> SDSLSKSPENWMSKLDDGKHLTEINIPGSHDSGSFTLKDPVKSVWAKTQDKDYLTQMKSGVRFFDIRGRASADNMISVHHGMVYLHHELGKFLDDAKYYLSAYPNETIVMSMKKDYDSDSKVTKTFEEIFREYYYNNPQYQNLFYTGSNANPTLKETKGKIVLFNRMGGTYIKSGYGADTSGIQWADNATFETKINNGSLNLKVQDEYKDYYDKKVEAVKNLLAKAKTDSNKDNVYVNFLSVASGGSAFNSTYNYASHINPEIAKTIKANGKARTGWLIVDYAGYTWPGYDDI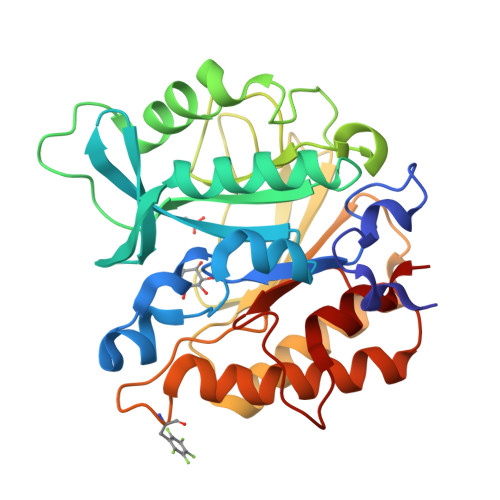VSEIIDSNK>MQTRTLEIGVGLFLLAGLLALLLLALRVSGLSVGNAGDTYKVYAYFDNIAGVTVRGKVTLAGVTIGKVTAVDLDRDSYTGRVTMEINQNVNNLPVDSTASILTAGLLGEKYIGISVGGDEDVLKDGSTIHDTQSALVLEDLIGKFLLNSVNKDEAKK[6x];>[2x]MRRVSPLERIRLFGRAGLDVVAALGRSTLFLGHALLGRRTPGTGLHLLVKQLYSVGVLSLAIIVVSGLFIGMVLALQGYNILISYGSEQAVGQMVALTLLRELGPVVTGLLFAGRAGSALTAEIGNMKATEQLSSLEMIGVDPLKYIVAPRLWAGFISMPLLAAIFSVVGIWGGAMVAVDWLGVYEGSFWANMQNSVQFTEDVLNGVIKSIVFAFVVTWIAVYQGYDCEPTSEGISRATTRTVVYASLAVLGLDFILTALMFGDF;>[2x]MSTDSAYAVELKGLTFKRGSRAIFDNIDVRIPRGKVTGIMGPSGCGKTTLLRLIASQLRPSKGEVWVNGQNLPQLSRGDLFDMRKQFGVLFQSGALFTDLDVFENVAFPLRVHTQLPEEMIRDIVLMKLQAVGLRGAVELMPDELSGGMKRRVALARAIALDPQILLYDEPFVGQDPIAMGVLVRLIRLLNDALGITSIVVSHDLAETASIADYIYIVGDGRVLGHGTPDVLKETDDPRIRQFVKGIPDGPVPFHYPARDYRADLLGER;>[2x]MSQASLREGAAGELQLAGVLDYSSGPALREQGGRLIRAS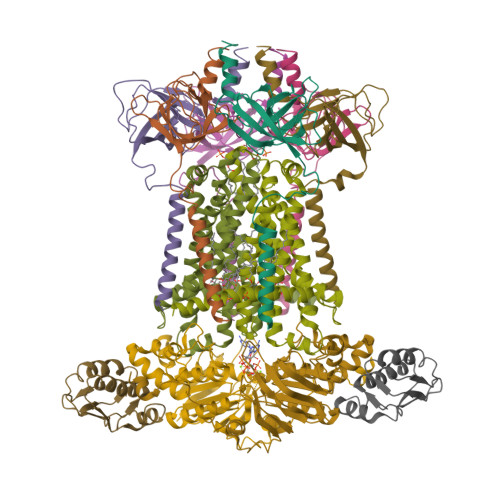QAAELVVDCSAVERSSSVGISLLLAFIRDARKAGKVLSVRALPDDMREIAKVSSLLEILPLQE N-methyl-N-({4-[4-(propan-2-yloxy)phenyl]-1H-pyrrol-3-yl}methyl)ethane-1,2-diamine | C17 H25 N3 O | 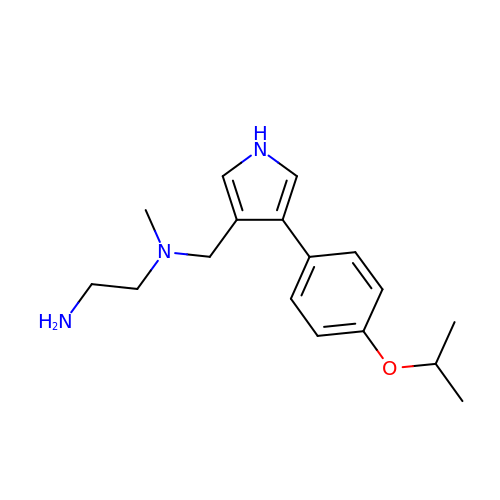FMTVWAGUJRUAKE-UHFFFAOYSA-N N-[(5-chloranyl-2-ethylsulfonyl-phenyl)methyl]-3-piperazin-1-yl-5-(trifluoromethyloxy)benzamide | C21 H23 Cl 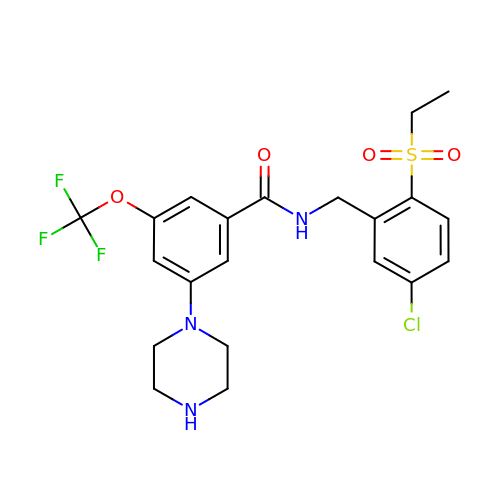F3 N3 O4 S | FNPFZOPPAGELAN-UHFFFAOYSA-N> GNYSVASNVMVPMRDGVRLAVDLYRPDADGPVPVLLVRNPYDKFDVFAWSTQSTNWLEFVRDGYAVVIQDTRGLFASEGEFVPHVDDEADAEDTLSWILEQAWCDGNVGMFGVSYLGVTQWQAAVSGVGGLKAIAPSMAS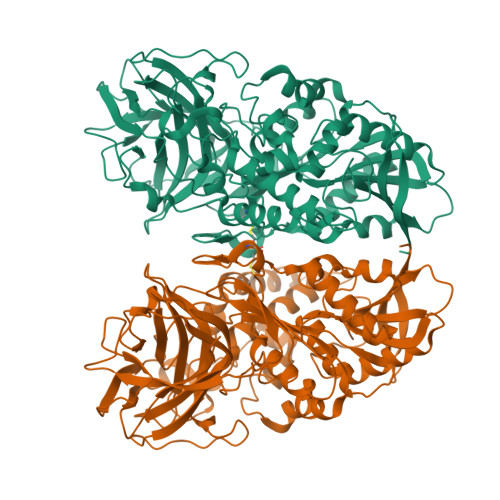ADLYRAPWYGPGGALSVEALLGWSALIGRQLITSRSDARPEDAADFVQLAAICNDVAGAASVTPLAEQPLLGRLIPWVIDQVVDHPDNDESWQSISLFERLGGLATPALITAGWYDGFVGESLRTFVAVKDNADARLVVGPWSHSNLTGRNADRKFGCAATYPIQEATTMHKAFFDRHLRGETDALAGVPKVRLFVMGIDEWRDETDWPLPDTAYTPFYLGGSGAANTSTGGGTLSTSISGTESADTYLYDPADPVPSLGGTLLFHNGDNGPADQRPIHDRDDVLCYSTEVLTDPVEVTGTVSARLFVSSSAVDTDFTAKLVDVFPDGRAIALCDGIVRMRYRETLVNPTLIEAGEIYEVAIDMLATSNVFLPGHRIMVQVSSSNFPKYDRNSNTGGVIAREQLEEMCTAVNRIHRGPEHPSHIVLPIIKR An adhesin from Mobiluncus mulieris, a bacterium associated with persistence in bacterial vaginosis, contains 51 repeat Ig-like domains. Each domain displays cross-linking including intramolecular ester, isopeptide, disulfide and thioester bonds. This giant 7651-residue protein, by far the largest in the bacterial proteome, is presumably retained because of its critical pathogenic role. The intramolecular cross-links, whether isopeptide or ester bonds, stabilize the individual Ig-like domains and provide a covalently linked ‘spine’ the entire length of the protein stretching from the surface of the bacterium to the adhesion domain.

Crystal structures of the mixed ester–isopeptide construct 46E–47I were solved in two different space groups. The molecules of the two space groups differ across 287 aligned Cα coordinates by a root-mean-square difference (r.m.s.d.) of 1.78 Å. Each pair of domains aligns more closely (Cα of residues 1–168, 0.72 Å r.m.s.d.; Cα of residues 169–292, 0.50 Å r.m.s.d.), suggesting that the flexible interdomain linker affords slightly different relative domain orientations. An unambiguous intramolecular ester-bond cross-link is seen to connect Thr6674 on the first β-strand of the domain fold to Gln6827 on the last β-strand. A short 2–3-amino-acid linker precedes the isopeptide-containing 47I domain. As predicted, an isopeptide bond links the first and last β-strands of this domain, joining Lys6842 to Asn6955. At the N-terminal end of the isopeptide domain 47I, the disulfide bond between Cys6895 and Cys6887 links two adjacent strands within the same β-sheet. The disulfide linkage between Cys6887 and Cys6895 identified by mass spectrometry in the 47I domain is not fully formed in the crystal structures, possibly as a result of radiation damage, and is consequently modelled at partial occupancy.

> KKPGVGTYATVDKLKAFDVTDGKKDAFTIKDTVRLYNVEEGKTYAIAGQLYEQSVAGDEGSALAKAATTVKVTASMAKPATEVEKTKYGEDVKVYETEMDLTVKREDLTKNQVVKDDIALVVYEQLWAEGTYEKVNDTEVTPKGKSEPVAKHNDPQSSSQSITAEPQFGSLKLTKTVTGWEDAFAKVARPEASYKFTVKCVQKGSVDEFTLKEGEEKTVEGIPLGDTCTISEDVQGAVNQAGLKDTVKFTAVNGVTVDSQVNGEAVVKIGGTANGSDTVANVEVTAENSFSY4-(4-methylpiperidin-1-yl)-N-(2-phenylethyl)pyrimidin-2-amine | C18 H24 N4 | 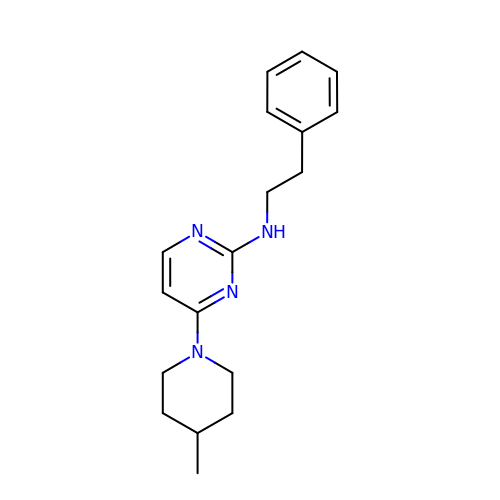FAHPWKWHSCNRBO-UHFFFAOYSA-N> KKQTQRNVFRCNVIGVKNCGKSGVLQALLGRNLMRQKKIREDHKSYYAINTVYVYGQEKYLLLHDISESEFLTEAEIICDVVCLVYDVSNPKSFEYCARIFKQHFMDSRIPCLIVAAKSDLHEVKQEYSISPTDFCRKHKMPPPQAFTCNTADAPSKDIFVKLTTMAMYPHVTQADLKSSTFLEHHHHHH

Human Miro1 and Miro2 (hMiro1, hMiro2, also called RhoT1 and RhoT2) are MOM protein homologs that play a critical role in mitochondrial trafficking38394041424344. Both associate with Parkin upon mitochondrial depolarization and are ubiquitinated on multiple lysines18374546. Here, we demonstrate that the cGTPase domain is necessary and sufficient for efficient ubiquitination of either hMiro1 or hMiro2 by p-S65 Parkin. We also find that despite considerable similarities between these two substrates, Parkin modifies hMiro1 much more robustly than hMiro2.

To better understand the difference in ubiquitination efficiency between hMiro1 and hMiro2, we first determined the crystal structures of the isolated cGTPase domains of both proteins to high resolution (hMiro1-C: 2.25 Å; hMiro2-C: 1.69 Å). The overall folds of the hMiro1 and hMiro2 cGTPase domains are quite similar (rmsd 0.78 Å over 129 Cα atoms). Unexpectedly, both domains crystallized as symmetric dimers. The dimer interface is a highly conserved hydrophobic surface along one face of the cGTPase domain, which, in the intact hMiro1-BC structure, forms the interface with the second hidden EF hand (hEF2). The cGTPase does not mediate dimerization in the context of the full-length molecule, as the hEF2/cGTPase interface is mutually exclusive with cGTPase dimerization, and hMiro1-BC is purely monomeric even at high concentrations. Interestingly, although the same conserved residues mediate dimerization in hMiro1-C and hMiro2-C, their dimer relationships differ significantly. We performed size exclusion chromatography with in-line multi-angle light scattering (SEC-MALS) and confirmed that both hMiro1-C and hMiro2-C dimerize in solution. Subsequently, we successfully disrupted dimerization of hMiro1-C in solution by introducing three mutations at the hydrophobic interface (V418R, Y470S, L472A), thereby generating a stable hMiro1 cGTPase monomer (hMiro1-CM). We note that the two lysines in addition to K572 identified as ubiquitinated by mass spectrometry of the hMiro1-CD, K454 and K512, can be mapped in the dimer, but not the monomer, to roughly the same continuous surface containing K572.> ELNRSQGIPFLEYKHFVTRTFFPKCSSLYEERYVLPSKTLNSQGGSPPQETHPLLGEWNIPEHCRPSMEEGISLFSSLLNNKHFLIVFVHALEQQKDFAVRDRCSLASLLTIALHGKLEYYTSIMKELLVDLIDASAAKNPKLMLRRTESVVEKMLTNWMSICMYGCLRETVGEPFFLLLCAIKQQINKGSIDAITGKARYTLNEEWLLRENIEAKPRNLNVSFQGCGMDSLSVRAMDTDTLTQVKEKILEAFCKNVPYSQWPRAEDVDLEWFASSTQSYVLRD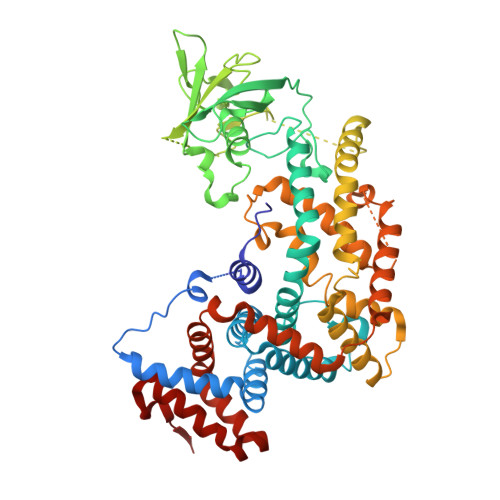LDDTSVVEDGRKKLNTLAHYKIPEGASLAMSLTDKKDSTLGRVKDLDTEKYFHLVLPTDELVEPKKSHRQSHRKKVLPEIYLTRLLSTKGTLQKFLDDLFKAILSIREDKPPLAVKYFFDFLEEQAEKRGISDPDTLHIWKTNSLPLRFWVNILKNPQFVFDIEKTDHIDACLSVIAQAFIDACSISDLQLGKDSPTNKLLYAKEIPEYRKTVQRYYKQIQDMTPLSEQEMNAHLAEESRKYQNEFNTNVAMAEIYKYAKRYRPQIMAALEANPTARRTQLQHKFEQVVALMENNIYECYSEA> GHMCIIKPMDDVVKFIHEVGSLKLTPRSGWLKLGIRLPESVAEHSFRAAIIAFILALKSGESVEKACKAATAALFHDLHEARTMDLHKIARRYVSCDEEGAREEQLSWMESKPDFSDVEVYVSDADKLELAFQGVEYSQQVSYAIRFAENVEL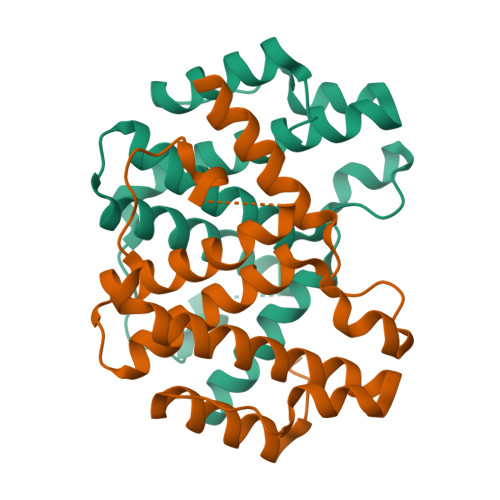KTDAAKEIYRVLMERKNPVWWR> QSAYSRIEAESYSNQSGIQTETCSEGGEDVGFVENGDYTVYNNVDFGDGVGGFQARVASATSGGNIEIRLDSSTGTLIGTCPVAGTGDWQTYTDAKCTVSGVTGKHDVYLVFKGDSGYL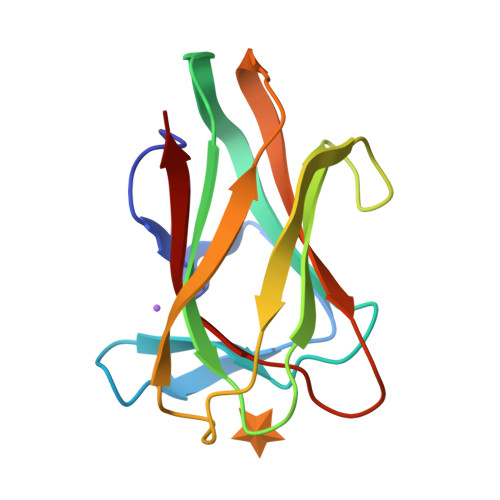FNLNWFTFSE> GAMEAMQKNELNSKIPIIFGLINSYQIHNLLEQHNAKTKESKAVFLIRDSSTYPGLLTISYYCQEQDIVKHIRFGLTDKGWKTAPKPPHEPLKSDSPEIKEKYTLDKIKFERKMKQFINTAKKLFEQHIRAESFKTLIMELKIHEFNLEGLI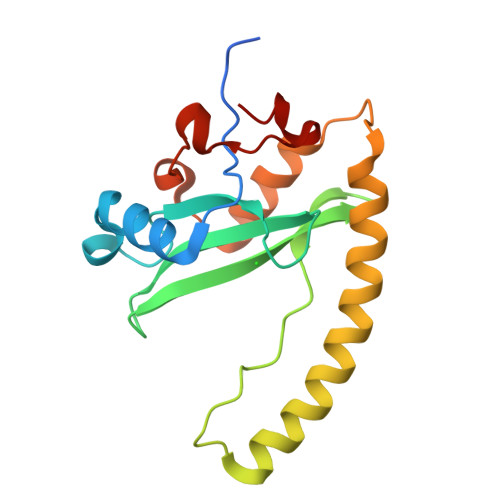KPTRSQASQEKHFTDYV>MGMEFSSHHIRLLQQLDEQRQKDLFCDCHIIVEGQMFKAHRNVLFASSGYFKMLLSQSCRDMGEPITATFDVFSADTFTAILD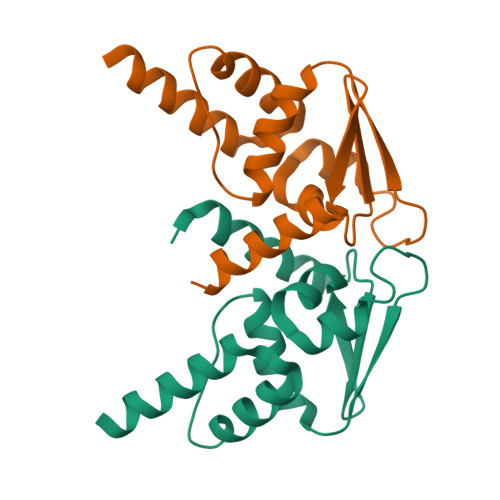FVYSGKLPLSGQNVIEVMSAADYLQMTDVIGVCKMFIKSSLDINEKDRDGFFSLSDKDAGSNGSGLEHHHHHH[6x]> AGGGGSSSGADHISLNPDLANEDEVNSCDYWRHCAVDGFLCSCCGGTTTTCPPGSTPSPISWIGTC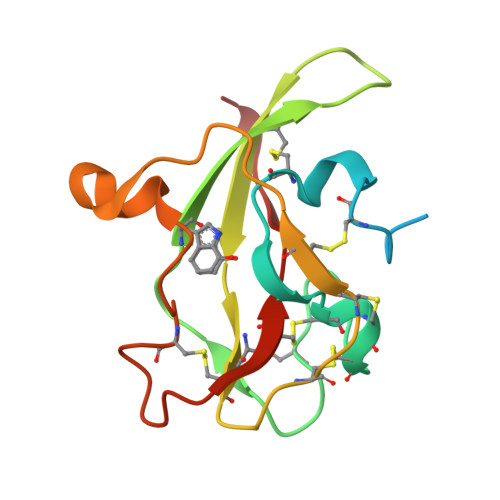HNPHDGKDYLISYHDCCGKTACGRCQCNTQTRERPGYEFFLHNDVNWCMANENSTFHCTTSVLVGLA> XXXXXXXXXXXXXXXXXXXXXXXXXXXXXXXXXXXXXXXXXXXXXXXXXXXXXXXXXXXXXXXXXXXXXXXXXXXXXXXXXXXXXXXXXXXXXXXXXXXXXXXXXXXXXXXXXXXXXXXXXXXXXXXXXXXXXXXXXXXXXXXXXXXXXXXXXXXXXXXXXXXXXXXXXXXXXXXXXXXXXXXXXXXXXXXXXXXXXXXXXXXXXXXXXXXXXXXXXXXXXXXXXXXXXXXXXXXXXXXXXXXXXXXXXXXXXXXXXXXXXXXXXXXXXXXXXXXXXXXXXXXXXXXXXXXXXXXXXXXXXXXXXXFSTNFRDTVDILVGWHIDHTQKPSLTQQVSGWLQSLEPFWVADLAFSTTLLGQFLEDMEAYAEDLSHVASGESVDEDVPPPSVSLPKLAALLRVFSTVVRSIGERFSPIRGPPITEAYVTDVLYRVMRCVTAANQVFFSEAVLTAANECVGVLLGSLDPSMTIHCDMVITYGLDQLENCQTCGTDYIISVLNLLTLIVEQINTKLPSSFVEKLFIPSSKLLFLRYHKEKEVVAVAHAVYQAVLSLKNIPVLETAYKLILGEMTCALNNLLHSLQLPEACSEIKHEAFKNHVFNVDNAKFVVIFDLSALTTIGNAKNSLIGMWALSPTVFALLSKNLMIVHSDLAVHFPAIQYAVLYTLYSHCTRHDHFISSSLSSSSPSLFDGAVISTVTTATKKHFSIILNLLGILLKKDNLNQDTRKLLMTWALEAAVLMRKSETYAPLFSLPSFHKFCKGLLANTLVEDVNICLQACSSLHALSSSLPDDLLQRCVDVCRVQLVHSGTRIRQAFGKLLKSIPLDVVLSNNNHTEIQEISLALRSHMSKAPSNTFHPQDFSDVISFILYGNSHRTGKDNWLERLFYSCQRLDKRDQSTIPRNLLKTDAVLWQWAIWEAAQFTVLSKLRTPLGRAQDTFQTIEGIIRSLAAHTLNPDQDVSQWTTADNDEGHGNNQLRLVLLLQYLENLEKLMYNAYEGCANALTSPPKVIRTFFYTNRQTCQDWLTRIRLSIMRVGLLAGQPAVTVRHGFDLLTEMKTTSLSQGNELEVTIMMVVEALCELHCPEAIQGIAVWSSSIVGKNLLWINSVAQQAEGRFEKASVEYQEHLCAMTGVDCCISSFDKSVLTLANAGRNSASPKHSLNGESRKTVLSKPTDSSPEVINYLGNKACECYISIADWAAVQEWQNSIHDLKKSTSSTSLNLKADFNYIKSLSSFESGKFVECTEQLELLPGENINLLAGGSKEKIDMKKLLPNMLSPDPRELQKSIEVQLLRSSVCLATALNPIEQDQKWQSITENVVKYLKQTSRIAIGPLRLSTLTVSQSLPVLSTLQLYCSSALENTVSNRLSTEDCLIPLFSEALRSCKQHDVRPWMQALRYTMYQNQLLEKIKEQTVPIRSHLMELGLTAAKFARKRGNVSLATRLLAQCSEVQLGKTTTAQDLVQHFKKLSTQGQVDEKWGPELDIEKTKLLYTAGQSTHAMEMLSSCAISFCKSVKAEYAVAKSILTLAKWIQAEWKEISGQLKQVYRAQHQQNFTGLSTLSKNILTLIELPSVNTMEEEYPRIESESTVHIGVGEPDFILGQLYHLSSVQAPEVAKSWAALASWAYRWGRKVVDNASXXXXXXXXXXXXXXXXXXXXXXXXXXXXXXXXXXXXXXXXXXXXXXXXXXXXXXXXXXXXXXXXXXXXXXXXXXXXXXXXXXXXXXXXEGVIKVWRKVVDRIFSLYKLSCSAYFTFLKLNAGQIPLDEDDPRLHLSHRVEQSTDDMIVMATLRLLRLLVKHAGELRQYLEHGLETTPTAPWRGIIPQLFSRLNHPEVYVRQSICNLLCRVAQDSPHLILYPAIVGTISLSSESQASGNKFSTAIPTLLGNIQGEELLVSECEGGSPPASQDSNKDEPKSGLNEDQAMMQDCYSKIVDKLSSANPTMVLQVQMLVAELRRVTVLWDELWLGVLLQQHMYVLXXXXXXXXXXXXXXXXXXXXXXXXXXXXXXXXXXXXXXXXXXXXXXXXXXXXXXXXPHEKWFQDNYGDAIENALEKLKXXXXXXXXXXXXXXXXXXXXXXXXXXXXXXXYILRLEEISPWLAAMTNTEIALPGEVSARDTVTIHSVGGTITILPTKTKPKKLLFLGSDGKSYPYLFKGLEDLHLDERIMQFLSIVNTMFATINRQETPRFHARHYSVTPLGTRSGLIQWVDGATPLFGLYKRWQQREAALQAQKAQDSYQTPQNPGIVPRPSELYYSKIGPALKTVGLSLDVSRRDWPLHVMKAVLEELMEATPPNLLAKELWSSCTTPDEWWRVTQSYARSTAVMSMVGYIIGLGDRHLDNVLIDMTTGEVVHIDYNVCFEKGKSLRVPEKVPFRMTQNIETALGVTGVEGVFRLSCEQVLHIMRRGRETLLTLLEAFVYDPLVDWTAGGEAGFAGAVYGGGGQQAESKQSKREMEREITRSLFSSRVAEIKVNWFKNRDEMLVVLPKLDGSLDEYLSLQEQLTDVEKLQGKLLEEIEFLEGAEGVDHPSHTLQHRYSEHTQLQTQQRAVQEAIQVKLNEFEQWITHYQAAFNNLEATQLASLLQEISTQMDLGPPSYVPATAFLQNAGQAHLISQCEQLEGEVGALLQQRRSVLRGCLEQLHHYATVALQYPKAIFQKHRIEQWKTWMEELICNTTVERCQELYRKYEMQYAPQPPPTVCQFITATEMTLQRYAADINSRLIRQVERLKQEAVTVPVCEDQLKEIERCIKVFLHENGEEGSLSLASVIISALCTLTRRNLMMEGAASSAGEQLVDLTSRDGAWFLEELCSMSGNVTCLVQLLKQCHLVPQDLDIPNPMEASETVHLANGVYTSLQELNSNFRQIIFPEALRCLMKGEYTLESMLHELDGLIEQTTDGVPLQTLVESLQAYLRNAAMGLEEETHAHYIDVARLLHAQYGELIQPRNGSVDETPKMSAGQMLLVAFDGMFAQVETAFSLLVEKLNKMEIPIAWRKIDIIREARSTQVNFFDDDNHRQVLEEIFFLKRLQTIKEFFRLCGTFSKTLSGSSSLEDQNTVNGPVQIVNVKTLFRNSCFSEDQMAKPIKAFTADFVRQLLIGLPNQALGLTLCSFISALGVDIIAQVEAKDFGAESKVSVDDLCKKAVEHNIQIGKFSQLVMNRATVLASSYDTAWKKHDLVRRLETSISSCKTSLQRVQLHIAMFQWQHEDLLINRPQAMSVTPPPRSAILTSMKKKLHTLSQIETSIATVQEKLAALESSIEQRLKWAGGANPALAPVLQDFEATIAERRNLVLKESQRASQVTFLCSNIIHFESLRTRTAEALNLDAALFELIKRCQQMCSFASQFNSSVSELELRLLQRVDTGLEHPIGSSEWLLSAHKQLTQDMSTQRAIQTEKEQQIETVCETIQNLVDNIKTVLTGHNRQLGDVKHLLKAMAKDEEAALADGEDVPYENSVRQFLGEYKSWQDNIQTVLFTLVQAMGQVRSQEHVEMLQEITPTLKELKTQSQSIYNNLVSFASPLVTDATNECSSPTSSATYQPSFAAAVRSNTGQKTQPDVMSQNARKLIQKNLATSADTPPSTVPGTGKSVACSPKKAVRDPKTGKAVQERNSYAVSVWKRVKAKLEGRDVDPNRRMSVAEQVDYVIKEATNLDNLAQLYEGWTAWV;> AKLLPPERMKHSIKLVDDQMNWCDSAIEYLLDQTDVLVVGVLGLQGTGKSMVMSLLSANTPEEDQRTYVFRAQSAEMKERGGNQTSGIDFFITQERIVFLDTQPILSPSILDHLINNDRKLPPEYNLPHTYVEMQSLQIAAFLFTVCHVVIVVQDWFTDLSLYRFLQTAEMVKPSTPSPSHESSSSSGSDEGTEYYPHLVFLQNKARREDFCPRKLRQMHLMIDQLMAHSHLRYKGTLSMLQCNVFPGLPPDFLDSEVNLFLVPFMDSEAESENPPRAGPGSSPLFSLLPGYRGHPSFQSLVSKLRSQVMSMARPQLSHTILTEKNWFHYAARIWDGVRKSSALAEYSRLLA

The PI3K-related kinase (PIKK) SMG1 monitors the progression of metazoan nonsense-mediated mRNA decay (NMD) by phosphorylating the RNA helicase UPF1. SMG1 is a member of the phosphatidylinositol-3-kinase-related kinase (PIKK) family, which also includes the ATM, ATR, DNA-PKc, and mTOR kinases. Despite the confounding name reflecting a possible evolutionary origin with a lipid kinase, and in retrospect the ability of some PIKK family members to bind inositol-6-phosphate, all active PIKKs are Ser-Thr protein kinases. These large, multidomain enzymes share an overall similar architecture: a C-terminal catalytic module (comprising the so-called FAT, kinase, and FATC domains) and an N-terminal α-solenoid (that typically serves as a protein-protein interaction module). SMG8 and SMG9 form an unusual G-domain heterodimer.

To address this question, we reconstituted purified wild-type SMG1-8-9 with an excess of AMPPNP (instead of SMG1i) and subjected the sample to a similar single-particle cryo-EM analysis routine. We obtained maps for SMG1-8-9 and SMG1-9 at overall resolutions of 2.8 Å and 3.1 Å, respectively (Figure 3—figure supplements 2 and 3). In the reconstruction of the binary SMG1-9 complex in the presence of AMPPNP, we observed no ordered density at the substrate-binding site, consistent with the reconstruction obtained in the presence of SMG1i. We concluded that the autoinhibitory conformation of the PRD in the insertion domain of SMG1 is connected to the presence of a nucleotide in the ATP-binding site and is stabilized by the presence of SMG8. In the binary SMG1-9 complex, the portion of SMG9 that interacts with the N-terminal HEAT repeat helices of SMG1 changes conformation, exploiting part of a binding site that was occupied by a short N-terminal segment of SMG8 in the ternary complex. Indeed, two hydrophobic residues of SMG9 (Leu456 and Leu457) take the place normally reserved for two hydrophobic residues of SMG8 (Leu351 and Leu352). Hence, the conformation of the SMG9 segment observed in the SMG1-9 complex is incompatible with the binding of SMG8 to this part of SMG1.>ADIQSFSFKNFNSSSFILQGDATVSSSKLRLTKVKGNGLPTLSSLGRAFYSSPIQIYDKSTGAVASWATSFTANIFAPNKSSSADGIAFALVPVGSEPKSNSGFLGVFDSDVYDNSAQTVAVEFDTFSNTDWDPTSRHIGIDVNSIKSIRTASWGLANGQNAEILITYNAATSLLVASLVHPSRRTSYIVSERVDITNELPEYVSI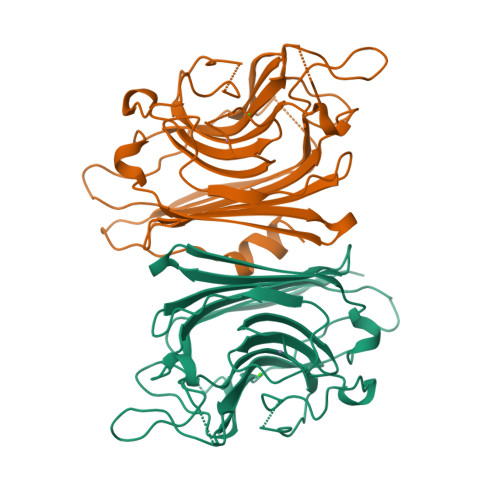GFSATTGLSEGYTETHDVLSWSFASKLPDDSTTEPLDIASYLVRNVL[6x]> ANHKNFILMLIILFLMEFARGMYILSYINFLPTVTSIAVAITSLAFSIHFIADASTNFVIGFLLKKFGTKIVLTTGFILAFTSLFLVIWFPASPFVIIFSAMMLGIAVSPIWVIMLSSVEEDKRGKQMGYVYFSWLLGLLVGMVFMNLLIKVHPTRFAFMMSLVVLIAWILYYFVDVKLTNYNTRPVKAQLRQIVDVTKRHLLLFPGILLQGAAIAALVPILPTYATKVINVSTIEYTVAIIIGGIGCAVSMLFLSKLIDNRSRNFMYGVILSGFILYMILIFTLSMIVNIHILWIIALAIGLMYGILLPAWNTFMARFIKSDEQEETWGVFNSIQGFGSMIGPLFGGLITQFTNNLNNTFYFSALIFLVLAV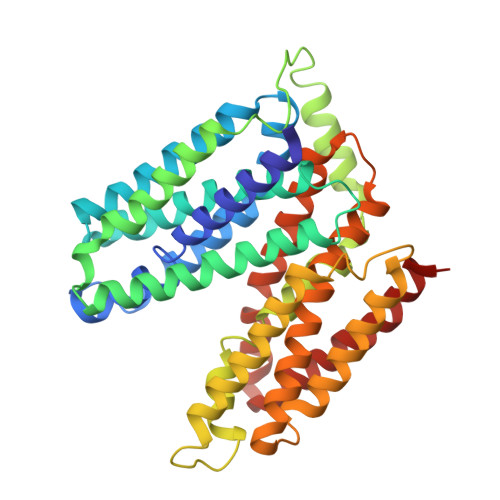FYGSY>[3x]GSHMLESKLQITPCGMLVQGNQINF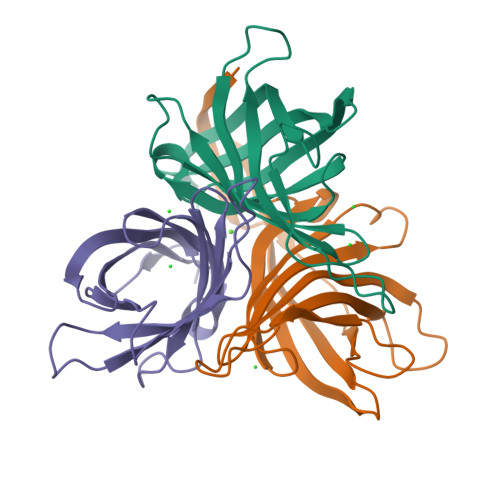TKLYLHHTPAGPEQNQSAVTSNDKKIGLGCIVVNNWSVYDGIGSDAKLVAYAKGLHVFAGAWHNSFSLVFEDERLKGSTLQVMGLIVEEGDWAIVGGTGQFAMATGVILKKMQEQKQYGNIIELTIHGFCPLLKGS> MCDLRRPAAGGMMDLAYVCEWEKWSKSTHCPSVPLACAWSCRNLIAFTMDLRSDDQDLTRMIHILDTEHPWDLHSIPSEHHEAITCLEWDQSGSRLLSADADGQIKCWSMADHLANSWESSVGSLVEGDPIVALSWLHNGVKLALHVEKSGASSFGEKFSRVKFSPSLTLFGGKPMEGWIAVTVSGLVTVSLLKPSGQVLTSTESLCRLRGRVALADIAFTGGGNIVVATADGSSASPVQFYKVCVSVVSEKCRIDTEILPSLFMRCTTDLNRKDKFPAITHLKFLARDMSEQVLLCASSQTSSIVECWSLRKEGLPVNNIFQQISPVVGDKQPTILKWRILSATNDLDRVSAVALPKLPISLTNTDLKVASDTQFYPGLGLALAFHDGSVHIVHRLSLQTMAVFYSSAAPRPVDEPAMKRPRTAGPAVHLKAMQLSWTSLALVGIDSHGKLSVLRLSPSMGHPLEVGLALRHLLFLLEYCMVTGYDWWDILLHVQPSMVQSLVEKLHEEYTR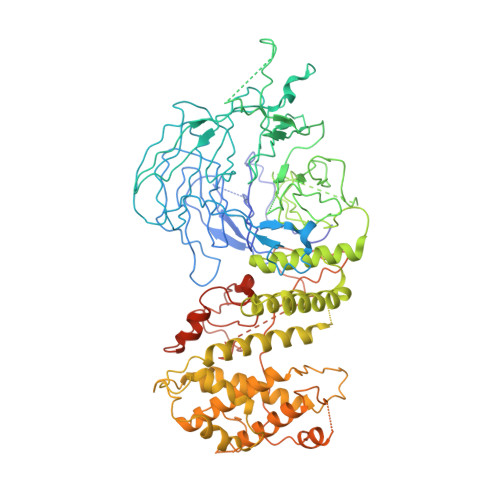QTAALQQVLSTRILAMKASLCKLSPCTVTRVCDYHTKLFLIAISSTLKSLLRPHFLNTPDKSPGDRLTEICTKITDVDIDKVMINLKTEEFVLDMNTLQALQQLLQWVGDFVLYLLASLPNQGSLLRPGHSFLRDGTSLGMLRELMVVIRIWGLLKPSCLPVYTATSDTQDSMSLLFRLLTKLWICCRDEGPASEPDEALVDECCLLPSQLLIPSLDWLPASDGLVSRLQPKQPLRLQFGRAPTLPGSAATLQLDGLARAPGQPKIDHLRRLHLGACPTEECKACTRCGCVTMLKSPNRTTAVKQWEQRWIKNCLAVEGRGPDACVTSRASEEAPAFVQLGPQSTHHSPRTPRSLDHLHPEDRP Human gamma-D crystallin (HGD) is a soluble, monomeric protein expressed in the eye lens during fetal development. The high expression levels contribute to the refractive index within the lens which focuses visible light upon the retina. However, this halts further expression of HGD. This means HGD must remain correctly folded and soluble for the entire human lifespan in order to maintain visual acuity. In order to observe structural changes in HGD, we take advantage of an arginine-to-serine point mutation, R36S, first identified in congenital cataracts (HGDm).

UV-lability of the Cys-DTT disulfide was tested by exposing similarly aged crystals to a UV LED at 285 nm during X-ray data collection. In the first 5 ms dataset, DTT adduct cleavage is visible at C41 and C108 in both chains, with oxidation to sulfenic acid observed at C41 in both chains. We show that UV exposure is then able to disrupt the disulfide bond, and partially restore the conformation to that of fresh crystallin. However, with continuous illumination we observe the formation of sulfenic acid at C41, cysteine at C108 and no obvious changes to the structure of the neighboring tryptophans W42 and W130 in both copies of HGDm in the asymmetric unit. No evidence of these modifications was observed in the electron density of the light structure nor was it possible to locate the liberated DTT. The analysis of atomic coordinate-derived conformational space (RoPE, described in Methods Section 4.6), show that while aging of the crystal produces a large shift in the conformational space, this is partially reversed by UV exposure. The corresponding interatomic distance plots also show a reversal of the conformational changes that occurred during aging for each chain. However, total reversal is precluded perhaps due to the rate of structural relaxation and oxidation of C41 to sulfenic acid, although a much smaller covalent modification, may continue to influence the conformation. In support of this, we have shown that after UV illumination of aged crystals, HGDm returns at least in part to the original conformational state of fresh protein. Hence, disulfide cleavage likely proceeds in the most part via tryptophan excitation.

>MKHHHHHHQGKITLYEDRGFQGRHYECSSDHPNLQPYLSRCNSASVDSGCWMLYEQPNYSGLQYFLRRGDYADHQQWMGLSDSVRSCRLIPHSGSHRIRLYEREDYRGQMIEFTEDCSCLQDRFRFNEIHSLNVLEGSWVLYELSNYRGRQYLLMPGDYRRYQDWGATNARVGSLRRVIDFS[2x]>[2x]MDKLLLHVGPTTIKEDVLVAGLENNVGFTSKEFVEALAYSLKGLRYVMGASKNYQPLIIPGGGTSAMESVTSLLKPNDKILVVSNGVFGDRWEQIFKRYPVNVKVLRPSPGDYVKPGEVEEEVRKSEYKLVALTHVETSTGVREPVKDVINKIRKYVELIVVDGVSSVGAEEVKAEEWNVDVYLTASQKALGSAAGLGLLLLSPKALSILDSQNSIAGYYLDLRNWLPVMRGAEEGKA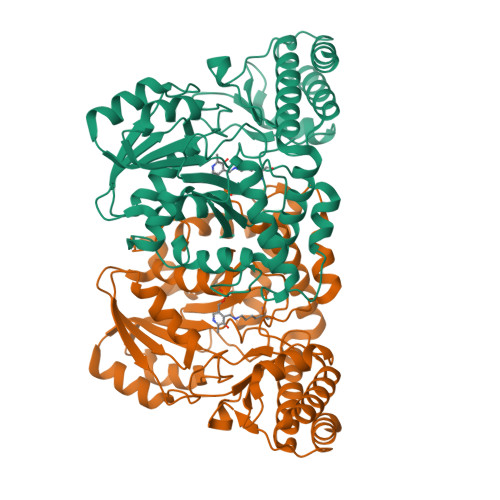AYFATPPVHVILQLAEAFRLIEKEGIENRIKRHTMVASAIRAGLEALGLEIVARRPESYSNTVTGVILKVADPQKVLAGTVNEGVEFAPGVHPAFKYFRIGHMGWVTPNDAIIAISVIERTLRKLGEPIRFGEGVKAVEEVLFSAR>[2x]TNYCNLQSCKRNNAIHTMCQYTSPTPGPMCLEYSNVGFTDAEKDAIVNKHN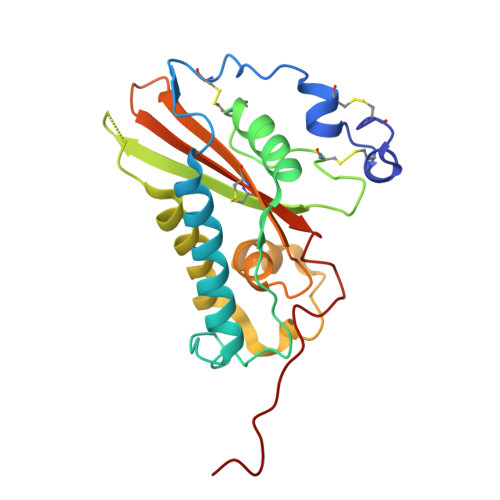ELRQRVASGKEMRGTNGPQPPAVKMPNLTWDPELATIAQRWANQCTFEHDACRNVERFAVGQNIAATSSSGKNKSTPNEMILLWYNEVKDFDNRWISSFPSDDNILMKVGHYTQIVWAKTTKIGCGRIMFKEPDNWTKHYLVCNYGPAGNVLGAPIYEIKKHHHHHH>[2x]MCGGLHRDGTPAGPSAGCPRLTAAALSAGQDALGPSSETQELECALDFLR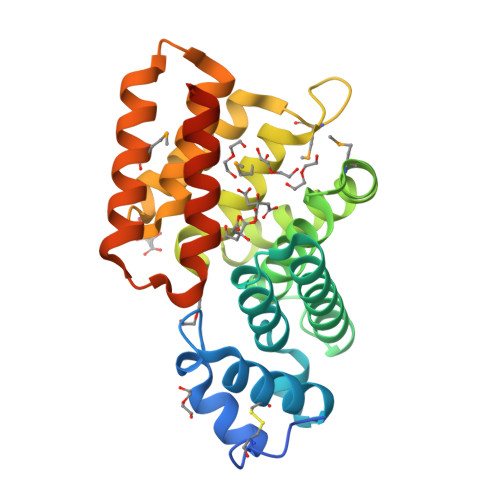GSDDPALRRSSLGSRICLHLAERNSDPAERARFAREGVERAEAALAQGGEDDGAVHYYLAANLGLAVRDDMTAALANLHRLEHESEAAVKLSPDFDDGGPLRLLGMLYLKAPAWPAGMGDGDKALDLLGQAVERHPGHPLNHLFYAEALWEVNGESESRRVEEEMAAGWRLLESGSWGYNKQIWKREFADLRQEIGAPARLEHHHHHH> ADPFKVLQEPTCVSDYMSISTCEWKMNGPTQCSTELRLLYQLVFLLSEAHTCIPENNGGAGCVCHLLMDDVVSADQYTLDLWAGQQLLWKGSFKPSEHVKPRAPGNLTVHTQVSDTLLLTWSNPYPPDNYLYNHLTYAVN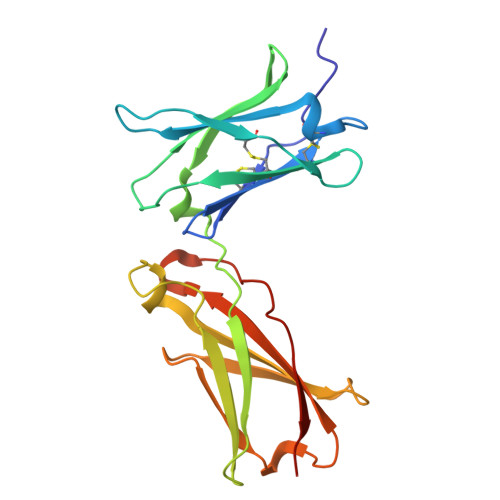IWSENDPADFRIYQVTYLEPSLRIAASTLKSGISYRARVRAWAQCYNTTWSEWSPSTKWHNSYRE> GSHMASPNGQTKPLPALKLALEYIVPCMNKHGICVVDDFLGKETGQQIGDEVRALHDTGKFTDGQLVSQKSDSSKDIRGDKITWIEGKEPGCETIGLLMSSMDDLIRHCNGKLGSYKINGRTKAMVACYPGNGTGYVRHVDNRNGDGRCVTCIYYLNKDWDAKVSGGILRIFPEGKAQFADIEPKFDRLLFFWSDRRNPHEVQPAYATRYAITVWYFDADERARAKVKYLTGEKGVRVELNKPSDSVGKDVF

The ferrous iron and 2-oxoglutarate (2OG)-dependent HIF prolyl hydroxylases (PHDs/EGLNs) catalyse trans-4-prolyl hydroxylations on HIFα subunits, thus promoting their binding to the von Hippel–Lindau protein (VHL), a targeting component of a ubiquitin E3 ligase, and signalling for HIFα degradation under normoxic conditions. The PHD-catalysed hydroxylations of HIF-1α/HIF-2α in higher animals occur in amino- and carboxy-terminal oxygen-dependent degradation domains (NODD and CODD). The three human PHDs exhibit different NODD/CODD selectivities, with PHD3 being substantially more selective for CODD than PHD1/2 (refs 16). Biophysical analyses employing crystallography and NMR reveal that the molecular basis of PHD isoform and variant selectivity involves enzyme–substrate interactions involving β2/β3 loop residues (that bind the LXXLAP motif) and helices α3 and α4, regions which display sequence variations between the PHD isoforms.

Analysis of a PHD2.N-oxalyl glycine (NOG).CODD complex structure led us to propose that certain erythrocytosis-associated PHD2 variants (P317R and R371H) would have altered substrate selectivities. Indeed, recombinant P317R PHD2 retains full CODD activity compared with wt PHD2, but strikingly does not hydroxylate NODD, suggesting its phenotype could be associated with loss of NODD hydroxylation. Structures of the P317R, R371H and R396T variants with a clinically used inhibitor628 reveal similar overall folds to wt PHD2, that is, a modified double-stranded-β-helix (DSBH) core (β-strands I–VIII), supporting 2OG and His-X-Asp…His-mediated Fe(II) binding. The structures suggested that these variants probably manifest altered substrate binding, but do not explain how their differing NODD/CODD selectivities arise. Comparison of the structures rationalizes the selectivities of the clinically observed P317R, R371H and R396T variants. Pro317PHD2 (βII-III loop) forms part of a hydrophobic patch binding the ODD LXXLAP-310-helix. The P317R structure reveals Arg317PHD2 present in two conformations, one predicted to interact differently with the LXXLAP motif. The lack of reactivity of P317R PHD2 with NODD supports a relatively more important role for Pro317PHD2 in binding the LXXLAP residues in NODD than CODD. P317R (which does not hydroxylate NODD, 2b) differs in that both inhibitors displace CODD to <10%, which is also less than for wt (with FG4592).>[3x]MAHHHHHHSSGLEVLFQGPMTHSVVELIEIESAIIQVKMQDRTHKNAFSQELTDDLIQAFEYIRQNPKYKAVILTGYDNYFASGGTQEGLLRIQQGLTAFTDDNLYSLALDCEIPVIAAMQGHGIGGGFVMGLFADIVILSRESVYTANFMKYGFTPGMGATFIVPKKLGFSLAQEILLNAGSYRGADLEKRGVPFKVLPRAEVLDYAVELAQELAEKPRNSLVTLKDHLVAPLRDQLPRVIEQELMMHE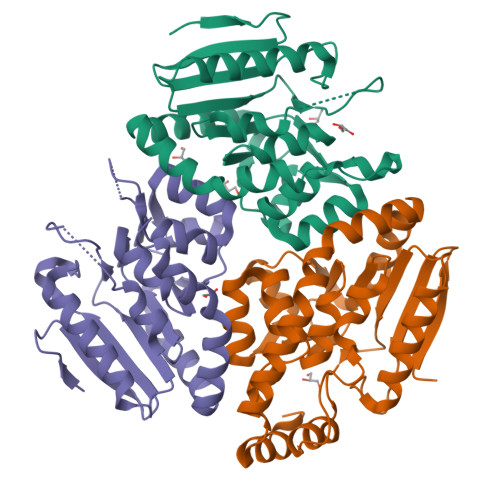KTFHHEEVKSRIKGLYGN>MEAVPRMPMIWLDLKEAGDFHFQPAVKKFVLKAAGENPEAYNEELKKLELLRQNAVRVPRDFEGCSVLRKYLGQLHYLQSRVPMGSGQEAAVPVTWTEIFSGKSVAHEDIKYEQACILYNLGALHSMLGAMDKRVSEEGMKVSCTHFQCAAGAFAYLREHFPQAYSVDMSRQILTLNVNLMLGQAQECLLEKSMLDNRKSFLVARISAQVVDYYKEACRALENPDTASLLGRIQKDWKKLVQMKIYYFAAVAHLHMGKQAEEQQKFGERVAYFQSALDKLNEAIKLAKGQPDTVQDALRFTMDVIGGKYNSAKKDNDFIYHEAVPALDTLQPVKGAPLVKPLPVNPTDPAVTGPDIFAKLV[2x];>LNVKVLEALELYNKLVNEAPV[2x]

HD-PTP is a non-receptor type protein tyrosine phosphatase (PTP) that contains five domains (Bro1, V, central proline-rich, PTP and second proline-rich domain). Considerable evidence has also indicated that HD-PTP and Myopic, the homologue of HD-PTP in Drosophila melanogaster, are involved in the morphogenesis of MVBs and in the endosomal sorting of cargo proteins, including integrin, Wntless and Wingless, and EGFR, and that the Bro1 domain is necessary for these processes. Thus far, two ESCRT components have been found to interact with the Bro1 domain of HD-PTP: the ESCRT-0 protein signal-transducing adaptor molecule 2 (STAM2) and the ESCRT-III protein charged multivesicular body protein 4B (CHMP4B). A recent report indicated that HD-PTP is the central regulator of EGFR sorting that functions to coordinate the transfer of EGFR from STAM2-containing ESCRT-0 to CHMP4B-containing ESCRT-III.

Herein, we identified that the residues 350–370 of STAM2 are necessary and sufficient for directly binding the Bro1 domain of HD-PTP, and determined the structure of the complex to a resolution of 2.0 Å. Therefore, with the expectation of altering crystal packing and promoting crystallization in a STAM2-bound form, we prepared a mutant HD-PTP(1–361) protein in which Asn33 and Tyr34 are substituted for alanine (referred to as HD-PTP(1–361;NAYA)). This mutant protein binds STAM2(350–370) as potently as the wild-type protein; this was confirmed using ITC. After incubation at a molar ratio of 1:5 between HD-PTP(1–361;NAYA) and the STAM2(350–370) peptide overnight, we crystallized the protein sample and obtained novel crystals with the space group P21 containing two HD-PTP molecules in the asymmetric unit. In the HD-PTP(1–361;NAYA)−STAM2(350–370) complex structure, the STAM2 peptide forms an amphipathic α-helix that binds to HD-PTP, mainly through hydrophobic interaction. In detail, the intermolecular hydrophobic interactions involve Val354, Leu358, Tyr361, Leu364 and Val365 of STAM2 and Leu189, Leu202, Ile206, Ala336, Leu338 and the hydrocarbon portions of Lys141, Lys192, and Arg198 of HD-PTP. Specifically, Tyr361 of STAM2 is located at the center of the hydrophobic cluster, suggesting that this residue plays a key role in the complex formation. Alanine substitution of this residue completely abrogated the binding interaction between the two proteins, as confirmed by ITC measurements. Along with the hydrophobic interactions, we note that hydrogen bonds mediated by three water molecules also reinforce the intermolecular binding between HD-PTP and STAM2. Intriguingly, we found that the STAM2 residues 351–353 play a key role in determining the binding partner of the protein; in the superposed models, this region brings about steric hindrance with the side chains of Lys151 of Alix and Arg145 of Brox, but not with that of the corresponding residue Thr145 of HD-PTP.>MASWSHPQFEKGSMRDIVDPVFSIGISSLWDELRHMPAGGVWWFNVDRHEDAISLANQTIASQAETAHVAVISMDSDPAKIFQLDDSQGPEK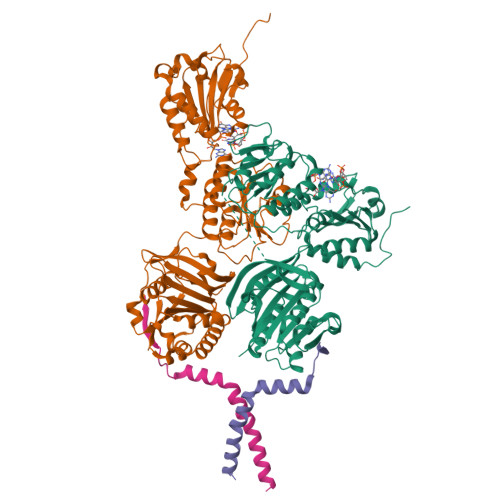IKLFSMLNHEKGLYYLTRDLQCSIDPHNYLFILVCANNAWQNIPAERLRSWLDKMNKWSRLNHCSLLVINPGNNNDKQFSLLLEEYRSLFGLASLRFQGDQHLLDIAFWCNEKGVSARQQLSVQQQNGIWTLVQSEEAEIQPRSDEKRILSNVAVLEGAPPLSEHWQLFNNNEVLFNEARTAQAATVVFSLQQNAQIEPLARSIHTLRRQRGSAMKILVRENTASLRATDERLLLACGANMVIPWNAPLSRCLTMIESVQGQKFSRYVPEDITTLLSMTQPLKLRGFQKWDVFCNAVNNMMNNPLLPAHGKGVLVALRPVPGIRVEQALTLCRPNRTGDIMTIGGNRLVLFLSFCRINDLDTALNHIFPLPTGDIFSNRMVWFEDDQISAELVQMRLLAPEQWGMPLPLTQSSKPVINAEHDGRHWRRIPEPMRLLDDAVERSS[2x];>[2x]MMTISDIIEIIVVCALIFFPLGYLARHSLRRIRDTLRLFFAKPRYVKPAGTLRRTEKARATKK>GPSSPMAGLEVLFASAAPAITCRQDALVCFLHWEVVTHGYCGLGVGDQPGPNDKKSELLPAGWNNNKDLYVLRYEYKDGSRKLLVKAITVESSMILNVLEYGSQQVADLTLNLDDYIDAEHLGDFHRTYKNSEELRSRIVSGIITPIHEQWEKANV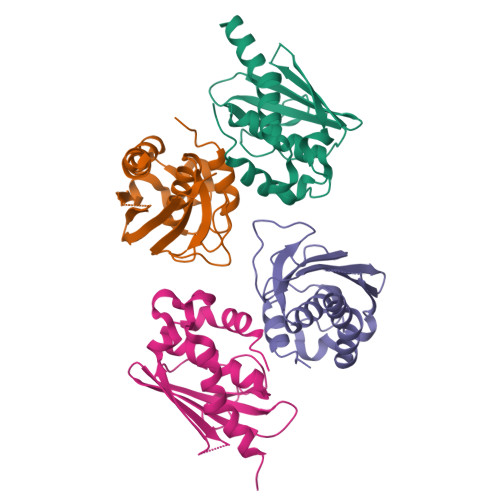SSPHREF[4x]>GGDNSVFDIFELTGAARKGSGRRLVKGPDPSSPAFRIEDANLIPPVPDDKFQDLVDAVRTEKGFLLLASLRQMKKTRGTLLALERKDHSGQVFSVVSNGKAGTLDLSLTVQGKQHVVSVEEALLATGQWKSITLFVQEDRAQLYIDCEKMENAELDVPIQSVFTRDLASIARLRIAKGGVNDNFQGVLQN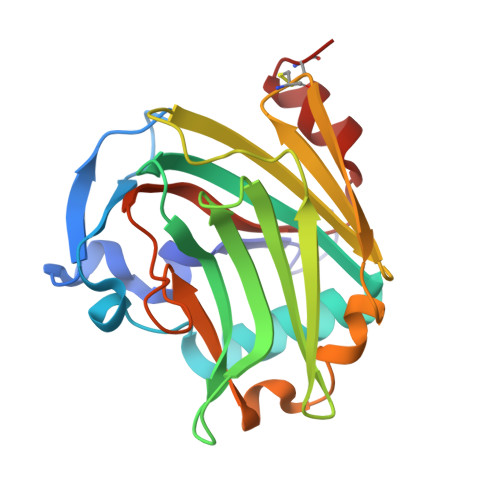VRFVFGTTPEDILRNKGCS[2x]> RLGE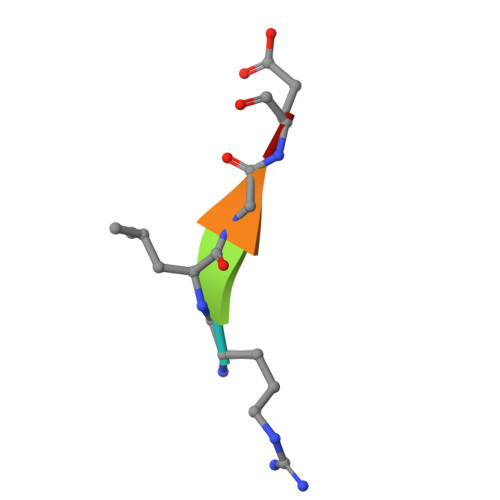S[(2-oxo-1,2-dihydroquinolin-4-yl)methyl]phosphonic acid | C10 H10 N O4 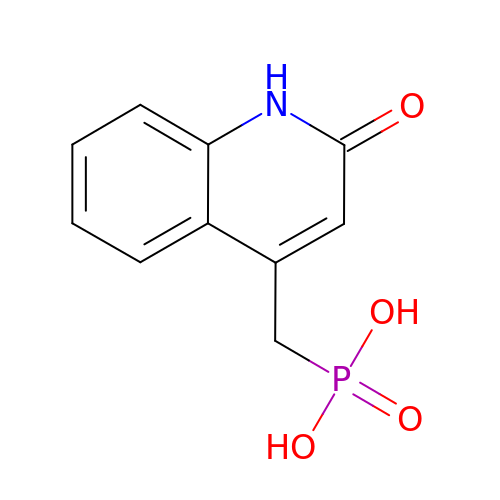P | KAIABXRDJQYKQE-UHFFFAOYSA-N> GLIVDTRDVEERVHVMRKTKLAPTVAHGVFNPEFGPAALSNKDSRLNEGVVLDEVIFSKHKGDTKMSAEDKA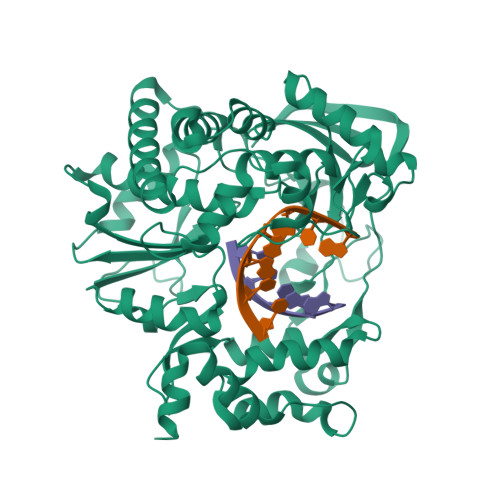LFRRCAADYASRLHSVLGTANAPLSIYEAIKGVDGLDAMEPDTAPGLPWALQGKRRGALIDFENGTVGPEVEAALKLMEKREYKFACQTFLKDEIRSMEKVRAGKTRIVDVLPVEHILYTRMMIGRFCAQMHSNNGPQIGSAVGCNPDVDWQRFGTHFAQYRNVWDVDYSAFDANHCSDAMNIMFEEVFRTEFGFHPNAEWILKTLVNTEHAYENKRITVEGGIPSGCSATSIINTILNNIYVLYALRRHYEGVELDTYTMISYGDDIVVASDYDLDFEALKPHFKSLGQTITPADKSDKGFVLGHSITDVTFLKRHFHMDYGTGFYKPVMASKTLEAILSFARRGTIQEKLISVAGLAVHSGPDEYRRLFEPFQGLFEIPSYRSLYLRWVNAVCGDAAALAHHHHHHH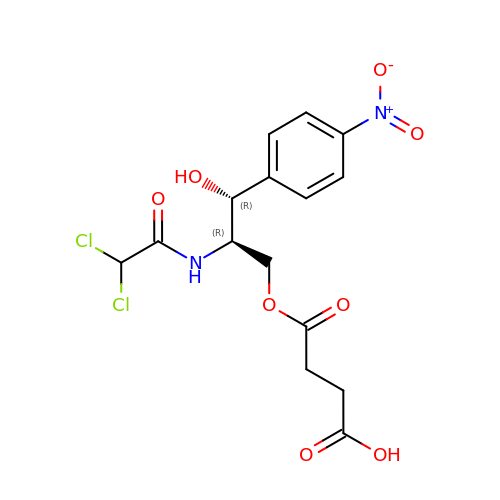CHLORAMPHENICOL SUCCINATE | C15 H16 Cl2 N2 O8 | LIRCDOVJWUGTMW-ZWNOBZJWSA-N>MEIAFLLNGETRRVRIEDPTQSLLEWLRAEGLTGTKEGCNEGDCGACTVMIRDAAGSRAVNACLMMLPQIAGKALRTIEGIAAPDGRLHPVQQAMIDHHGSQCGFCTPGFIVSMAAAHDRDRKDYDDLLAGNLCRCTGYAPILRAAEAAAGEPPADWLQADAAFTLAQLSSGVRGQTAPAFLPETSDALADWYLAHPEATLIAGGTDVSLWVTKALRDLPEVAFLSHCKDLAQIRETPDGYGIGAGVTIAALRAFAEGPHPALAGLLRRFASEQVRQVATIGGNIANGSPIGDGPPALIAMGASLTLRRGQERRRMPLEDFFLEYRKQDRRPGEFVESVTLPKSAPGLRCYKLSKRFDQDISAVCGCLNLTLKGSKIETARIAFGGMAGVPKRAAAFEAALIGQDFREDTIAAALPLLAQDFTPLSDMRASAAYRMNAAQAMALRYVRELSGEAVAVLEVMP[4x];>[4x]MSVGKPLPHDSARAHVT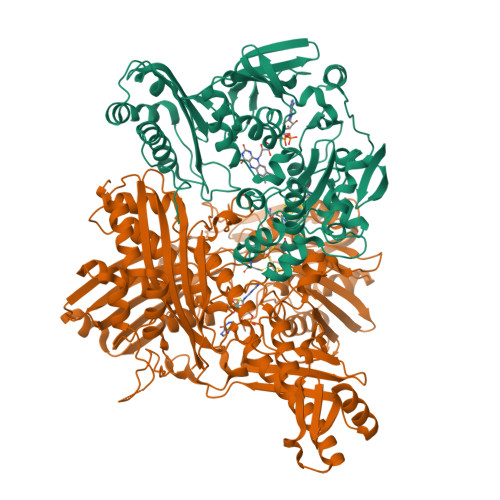GQARYLDDLPCPANTLHLAFGLSTEASAAITGLDLEPVRESPGVIAVFTAADLPHDNDASPAPSPEPVLATGEVHFVGQPIFLVAATSHRAARIAARKARITYAPRPAILTLDQALAADSRFEGGPVIWARGDVETALAGAAHLAEGCFEIGGQEHFYLEGQAALALPAEGGVVIHCSSQHPSEIQHKVAHALGLAFHDVRVEMRRMGGGFGGKESQGNHLAIACAVAARATGRPCKMRYDRDDDMVITGKRHDFRIRYRIGADASGKLLGADFVHLARCGWSADLSLPVCDRAMLHADGSYFVPALRIESHRLRTNTQSNTAFRGFGGPQGALGMERAIEHLARGMGRDPAELRALNFYDPPERGGLSAPPSPPEPIATKKTQTTHYGQEVADCVLGELVTRLQKSANFTTRRAEIAAWNSTNRTLARGIALSPVKFGISFTLTHLNQAGALVQIYTDGSVALNHGGTEMGQGLHAKMVQVAAAVLGIDPVQVRITATDTSKVPNTSATAASSGADMNGMAVKDACETLRGRLAGFVAAREGCAARDVIFDAGQVQASGKSWRFAEIVAAAYMARISLSATGFYATPKLSWDRLRGQGRPFLYFAYGAAITEVVIDRLTGENRILRTDILHDAGASLNPALDIGQIEGAYVQGAGWLTTEELVWDHCGRLMTHAPSTYKIPAFSDRPRIFNVALWDQPNREETIFRSKAVGEPPFLLGISAFLALHDACAACGPHWPDLQAPATPEAVLAAVRRAEGRA>GSHMNKKKAIFLFDVDGTLTISRKTIEQNVVDTLLELKSKKGFVLGIVGGSDYKKIREQIKYPEIFDYIFSENGVVAHKNDEEYFAESIVNFLGEDRLKKLINYSLKYIANLDIPKKRGTFIELRNGIINISPIGRNCSQEERDEFFRYNLKNNTIEKFRDNLSKEFEDFDLNFSMGGQISIDCFPKGWD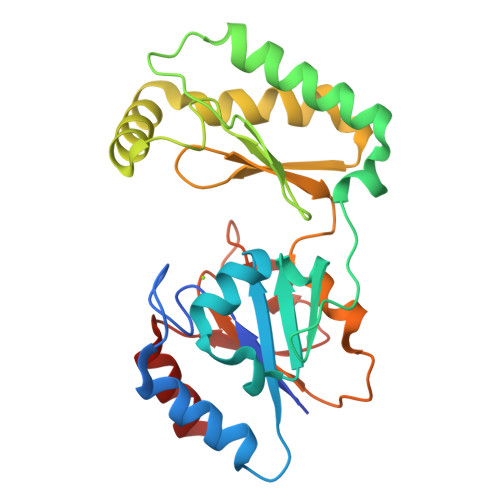KTFCLKHLENKFDEIYFFGDRTDKGGNDYELFCDKRVKGYKVKNPNDTVKILRENFL[2x]>GSNLEERLRACMQKLACGKLTGISDPVTVKTSGSRFGSWMTDPLAPEGDNRVWYMDGYHNNRFVREYKSMVDFMNTDNFTSHRLPHPWSGTGQVVYNGSIYFNKFQSHIIIR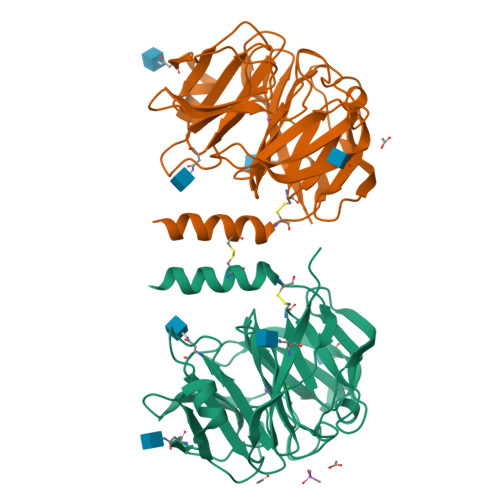FDLKTETILKTRSLDYAGYNNMYHYAWGGHSDIDLMVDENGLWAVYATNQNAGNIVISKLDPVSLQILQTWNTSYPKRSAGEAFIICGTLYVTNGYSGGTKVHYAYQTNASTYEYIDIPFQNKYSHISMLDYNPKDRALYAWNNGHQTLYNVTLFHAAAHHHHHH[2x]> MARIRHVQGDITEFQGDAIVNAANNYLKLGAGVAGAILRKGGPSIQEECDRIGKIRVGEAAVTGAGN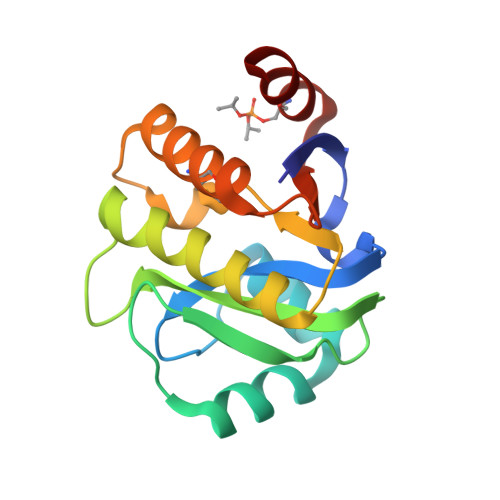LPVRYVIHAAVLGDEPASLETVRKATKSALEKAVELGLKTVAFTSWGAWVGGLPAEAVHRVMGEEIKKAPDTLEVTGVHGTEKSAEAYRRAS>GGGGIGVSTGTYDNQTTYKFLGDGWVEITAHASRLLHLGM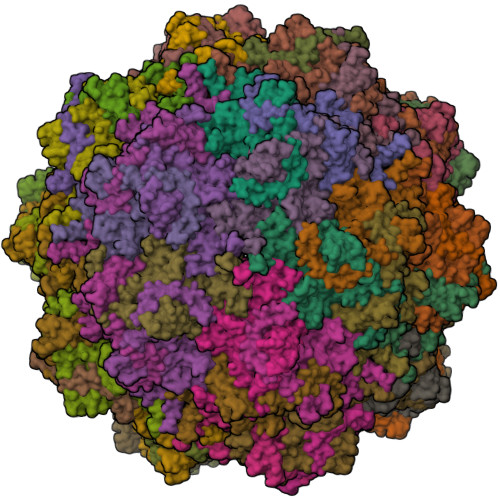PPSENYCRVTVHNNQTTGHGTKVKGNMAYDDTHQQIWTPWSLVDANAWGVWFQPSDWQFIQNSMESLNLDSLSQELFNVVVKTVTEQQGAGQDAIKVYNNDLTACMMVALDSNNILPYTPAAQTSETLGFYPWKPTAPAPYRYYFFMPRQLSVTSSNSAEGTQITDTIGEPQALNSQFFTIENTLPITLLRTGDEFTTGTYIFNTDPLKLTHTWQTNRHLGMPPRITDLPTSDTATASLTANGDRFGSTQTQNVNYVTEALRTRPAQIGFMQPHDNFEANRGGPFKVPVVPLDITAGEDHDANGAIRFNYGKQHGEDWAKQGAAPERYTWDAIDSAAGRDTARCFVQSAPISIPPNQNQILQREDAIAGRTNMHYTNVFNSYGPLSAFPHPDPIYPNGQIWDKELDLEHKPRLHVTAPFVCKNNPPGQLFVRLGPNLTDQFDPNSTTVSRIVTYSTFYWKGILKFKAKLRPNLTWNPVYQATTDSVANSYMNVKKWLPSATGNMHSDPLICRPVPHMTY[60x]>[2x]IVGGYICEENSVPYQVSLNSGYHFCGGSLISEQWVVSAGHCYKSRIQVRLGEHNIEVLEGNEQFINAAKIIRHPKYNSRTLDNDILLIKLSSPA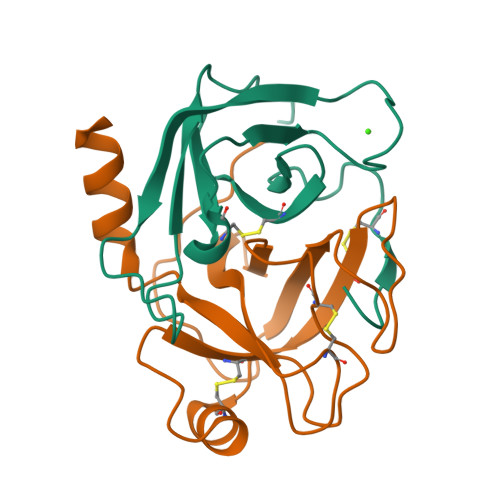VINSR;>[2x]VSAISLPTAPPAAGTESLISGWGNTLSSGADYPDELQCLDAPVLSQAECEASYPGKITNNMFCVGFLEGGKDSCQGDSGGPVVSNGELQGIVSWGYGCAQKNRPGVYTKVYNYVDWIKDTIAANS>GCACGCGC[2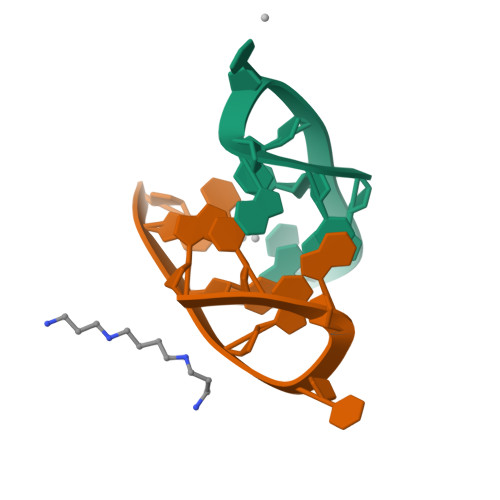x]> MGSSHHHH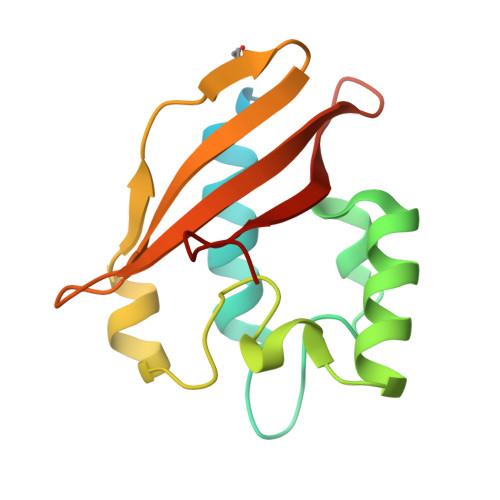HHENLYFQGHMGSAQAAVSQNSPEAAAISFYTWFIQHDSDQTYPLSEPDIERYVATDTVGRLRNDYAHAGPPNGVDYFLKVQDYDSRDWLAHIQVQRALMLGDVAVVPVSFGSQDPVHVLVFLKRVDATWKIIKIDDTWEYR> KVFSKCELAHKLKAQEMDGFGGYSLANWVCMAEYESNFNTRAFNGKNANGSSDYGLFQLNNKWWCKDNKRSSSNAC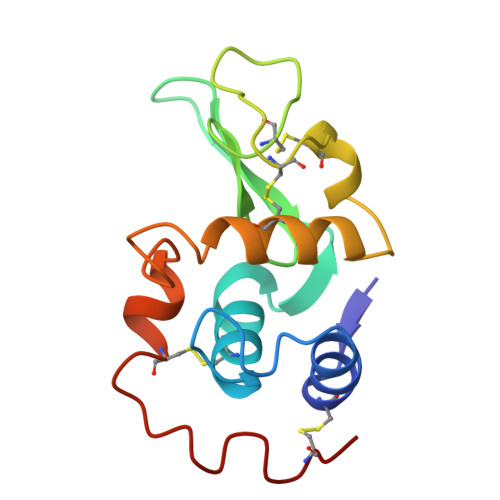NIMCSKLLDENIDDDISCAKRVVRDPKGMSAWKAWVKHCKDKDLSEYLASCNL2-(1H-indazol-1-yl)-N,N-dimethylacetamide 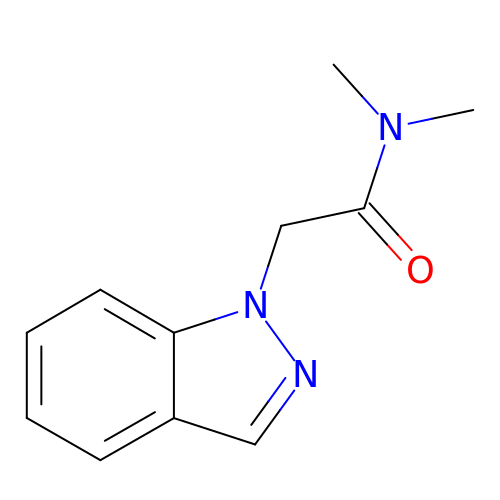| C11 H13 N3 O | AOLISVCNSODKGB-UHFFFAOYSA-N> MGHHHHHHAWNVYAYPKSEKERVPETTKEAYHFVLVPEELDNDYWRLVEKGAKAAAKELGVDLEYIGPRQANIDEHLRILKKAAAAKVDGIITQGLTEAEFVPVINEITDKNIPVVTIDTDAPTSRRVAYVGTDNYYAGFLAGRALAEDTKGKATVAIITGSLTAAHQQLRVRGFEDAVRQEKGIRIVAIEESHITRVQAAEKAYTILKKHPDVNAFYGTSALDAIGVAKVVEQFHREQKTYIIGFDTLPETIRYLQKGTIAATVV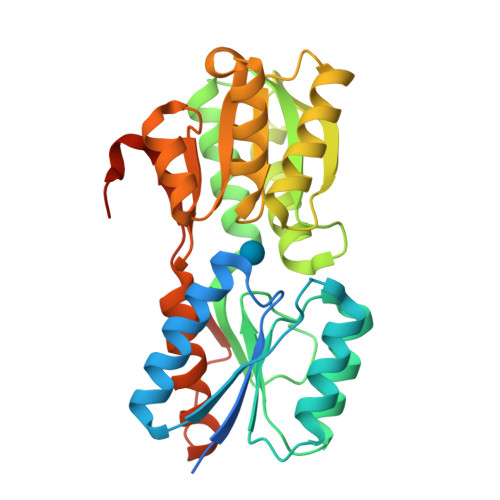QEPYEMGYKAVKMMAEIVAGKDVPVVTNTETKVIRKKDLPLRPARNYEVNTP> AADSARSFLERLEARGGREGAVLAGEFSDIQACSAAWKADGVCSTVAGSR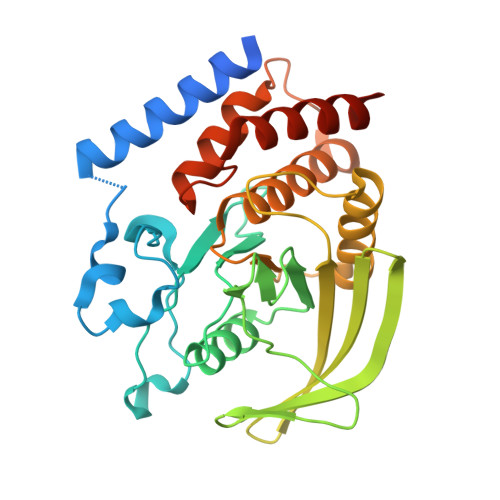PENVRKNRYKDVLPYDQTRVILSLLQEEGHSDYINGNFIRGVDGSLAYIATQGPLPHTLLDFWRLVWEFGVKVILMACREIENGRKRCERYWAQEQEPLQTGLFCITLIKEKWLNEDIMLRTLKVTFQKESRSVYQLQYMSWPDRGVPSSPDHMLAMVEEARRLQGSGPEPLCVHSSAGCGRTGVLCTVDYVRQLLLTQMIPPDFSLFDVVLKMRKQRPAAVQTEEQYRFLYHTVAQMFCSTLQNAS> MAGAQDFVPHTADLAELAAAAGECRGCGLYRDATQAVFGAGGRSARIMMIG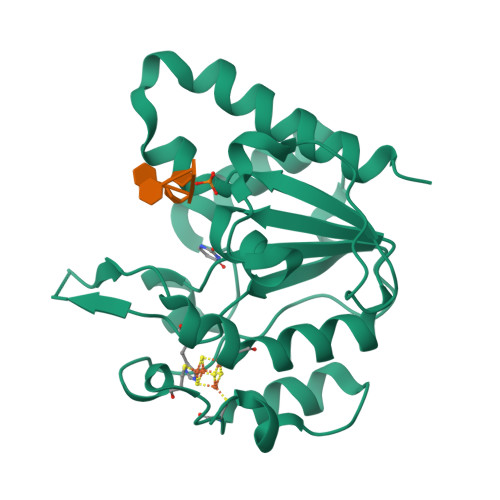EQPGDKEDLAGLPFVGPAGRLLDRALEAADIDRDALYVTNAVKHFKFTRAAGGKRRIHKTPSRTEVVACRPWLIAEMTSVEPDVVVLLGATAAKALLGNDFRVTQHRGEVLHVDDVPGDPALVATVHPSSLLRGPKEERESAFAGLVDDLRVAADVRP Tumour necrosis factor (TNF) is an important therapeutic target for treating a range of autoimmune and inflammatory disorders. TNF is a pleiotropic cytokine that exerts broad functional activity via binding and activation of two distinct receptors: TNF receptor 1 (TNFR1) and TNF receptor 2 (TNFR2). The small molecule compounds bind in a pocket at the centre of the TNF trimer and stabilise a conformation where a single TNF monomer subunit is perturbed, thereby inducing a molecular asymmetry in the trimer which in turn affects TNFR1 receptor interaction stoichiometry and subsequent signalling. To facilitate further characterisation of these small molecule compounds in a variety of contexts, we here generate a monoclonal antibody, known as CA1974, that selectively binds with high affinity to the TNF trimer–small molecule complex.

Structures of TNF in association with small-molecule indicate that the normally symmetric trimer becomes distorted, resulting in a breakdown in trimerous symmetry. A prominent feature of this perturbation is the generation of an expanded cleft at the altered interface between two of the monomer subunits (subunits A and C). Overall the homology was very high, with an RMSD = 0.43 Å with no significant variation in the degree of distortion at the A/C receptor binding interface. Variation was seen in loops containing Tyr87 (Fig. 4a red circles) but this is perhaps not unexpected, given that the loops are flexible and poorly ordered in the compound-only structure. Whereas in the structure with Fab and receptors the loops are stabilised through protein contacts with either receptors or Fab. This suggests that the CA1974 antibody recognises the true small molecule-stabilised form of the TNF trimer and does not induce significant further structural rearrangements as a result of binding.

>SVRSSSRTPSDKPVAHVVANPQAEGQLQWLNRRANALLANGVELRDNQLVVPSEGLYLIYSQVLFKGQGCPSTHVLLTHTISRIAVSYQTKVNLLSAIKSPCQRETPEGAEAKPWYEPIYLGGVFQLEKGDRLSAEINRPDYLDFAESGQVYFGIIAL[3x]>[7x]MNQRLMTGDAMQANFGFVTSQTAYVEAGVYRMRYPEIRYPGLIPVDYSAPEWIKTVDYYSMDGVG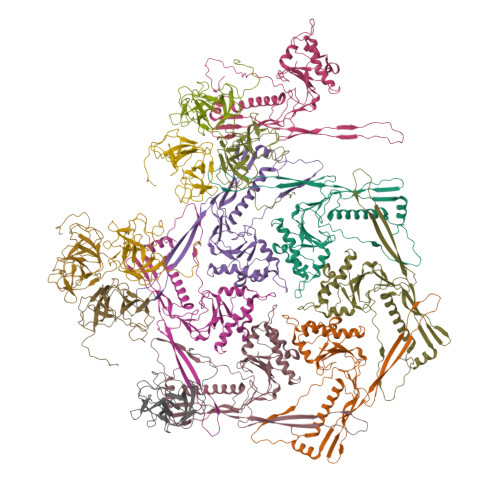KAEWIADRASDIPVVGLAMEKATTTVHLAGIGYDYGLEEVNQAIMLGMNLPGEKANLARLVYERMVDRVAFTGDAEKDFKGLFNNGAVTAVSATTGNWASATADQILADFNLGITGLWSATNEMVYADTVLLPSAKHQIIASKRLGNEATETVLQFLQRANVYTAETGRPLTIRGMRGLNTAGAGGVSRSVFYRNSPEVLKMHIPMRHRFLPVQVVGLTYKVPGIFRLGGLDIRLPKEVRYVDGY;>[7x]MAPYNETYASDYAFAYEGMVSDIAPADIISRTVETSAGIGFGKIVAQGTSDRGCKADVSAVSPTAPPLGITVRSQATENLTLDKYPRYDGAAIMRKGVIWVLVTDAGGVVAGDPVWLKKSDGTFSNADVGSSGGLRLAGCRWDTSAANGALARMRVDFDVPPVAGA>[2x]TDTTLPPDDSLDRIEPVDIEQEMQRSYIDYAMSVIVGRALPEVRDGLKPVHRRVLYAMFDSGFRPDRSHAKSARSVAETMGNYHPHGDASIYDSLVRMAQPWSLRYPLVDGQGNFGSPGNDPPAAMRYTEARLTPLAMEMLREIDEETVDFIPNYDGRVQEPTVLPSRFPNLLANGSGGIAVGMATNIPPHNLRELADAVFWALENHDADEEETLAAVMGRVKGPDFPTAGLIVGSQGTADAYKTGRGSIRMRGVVEVEEDSRGRTSLVITELPYQVNHDNFITSIAEQVRDGKLAGISNIEDQSSDRVGLRIVIEIKRDAVAKVVINNLYKHTQLQTSFGANMLAIVDGVPRTLRLDQLIRYYVDHQLDVIVRRTTYRLRKANERAHILRGLVKALDALDEVIALIRASETVDIARAGLIELLDIDEIQAQAILDMQLRRLAALERQRIIDDLAKIEAEIADLEDILAKPERQRGIVRDELAEIVDRHGDDRRTRIIAIDGDVSDEDLIAREDVVVTITETGYAKRTKTDLYRSQKRGGKGVQGAGLKQDDIVAHFFVCSTHDLILFFTTQGRVYRAKAYDLPEASRT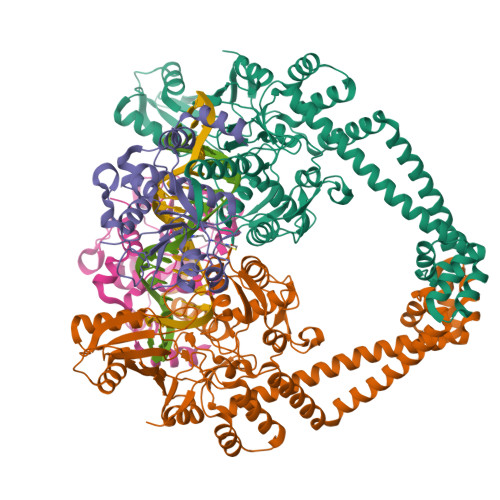ARGQHVANLLAFQPEERIAQVIQIRGYTDAPYLVLATRNGLVKKSKLTDFDSNRSGGIVAVNLRDNDELVGAVLCSAGDDLLLVSANGQSIRFSATDEALRPMGRATSGVQGMRFNIDDRLLSLNVVREGTYLLVATSGGYAKRTAIEEYPVQGRGGKGVLTVMYDRRRGRLVGALIVDDDSELYAVTSGGGVIRTAARQVRKAGRQTKGVRLMNLGEGDTLLAIARNAEESGDDNAVDANGADQTGN;>[2x]GAMVAAQKKKAQDEYGAASITILEGLEAVRKRPGMYIGSTGERGLHHLIWEVVDNAVDEAMAGYATTVNVVLLEDGGVEVADDGRGIPVATHASGIPTVDVVMTQLHAGGKFDSDAYAISGGLHGVGVSVVNALSTRLEVEIKRDGYEWSQVYEKSEPLGLKQGAPTKKTGSTVRFWADPAVFETTEYDFETVARRLQEMAFLNKGLTINLTDERVTQDEVVDEVVSDVAEAPKSASERAAESTAPHKVKSRTFHYPGGLVDFVKHINRTKNAIHSSIVDFSGKGTGHEVEIAMQWNAGYSESVHTFANTINTHEGGTHEEGFRSALTSVVNKYAKDRKLLKDKDPNLTGDDIREGLAAVISVKVSEPQFEGQTKTKLGNTEVKSFVQKVCNEQLTHWFEANPTDAKVVVNKAVSSAQARIAARKARELVRRKSATDIGGLPGKLADCRSTDPRKSELYVVEGDSAGGSAKSGRDSMFQAILPLRGKIINVEKARIDRVLKNTEVQAIITALGTGIHDEFDIGKLRYHKIVLMADADVDGQHISTLLLTLLFRFMRPLIENGHVFLAQPPLYKLKWQRSDPEFAYSDRERDGLLEAGLKAGKKINKEDGIQRYKGLGEMDAKELWETTMDPSVRVLRQVTLDDAAAADELFSILMGEDVDARRSFITRNAKDVRFLDV> TSDPVRQYLHEIGQVPLLTLEEEIDLARKVEEGMEAIKKLSEATGLDQELIREVVRAKILGTARIQKIPGLKEKPDPKTVEEVDGKLKSLPKELKRYLHIAREGEAARQHLIEANLRLVVSIAKKYTGRGLSFLDLIQEGNQGLIRAVEKFEYKRRFKFSTYATWWIRQAINRAIADQARTIRIPVHMVETINKLSRTARQLQQELGREPSYEEIAEAMGPGWDAKRVEETLKIAQEPVSLETPIGDEKDSFYGDFIPDENLPSPVEAAAQSLLSEELEKALSKLSEREAMVLKLRKGLIDGREHTLEEVG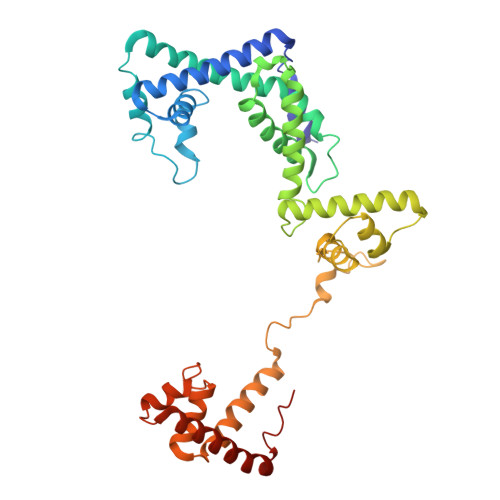AYFGVTRERIRQIENKALRKLKYHESRTRKLRDFLE>[12x]MAHHHHHHKDEVALLAAVTLLGVLLQAYFSLQVISARRAFRVSPPLTTGPPEFERVYRAQVNCSEYFPLFLATLWVAGIFFHEGAAALCGLVYLFARLRYFQGY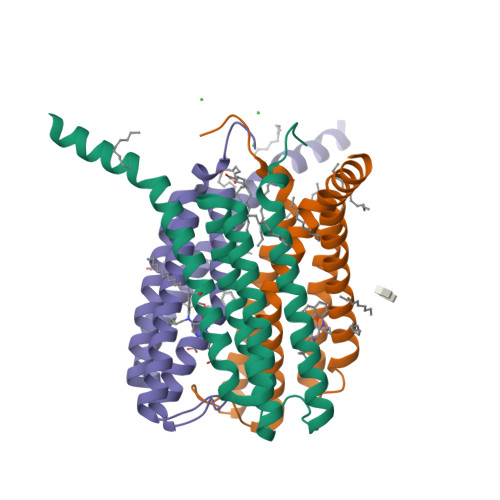ARSAQLRLAPLYASARALWLLVALAALGLLAHFLPAALRAALLGRLRTLLPWA>SSSTTLHNAMQYTAFDVLSSILNLMKADPLYDLLQLNQAYSSQDQEYEKNEFYGDSYLEERASSLVLKFLRKYEQIPFEMYSGLRIHTVKNQTLGEIFDLLHLGDTKTFEKKKKGDLVESLIGGCVLLSQRENATLFLLFAHALIDYIFYHSSYIY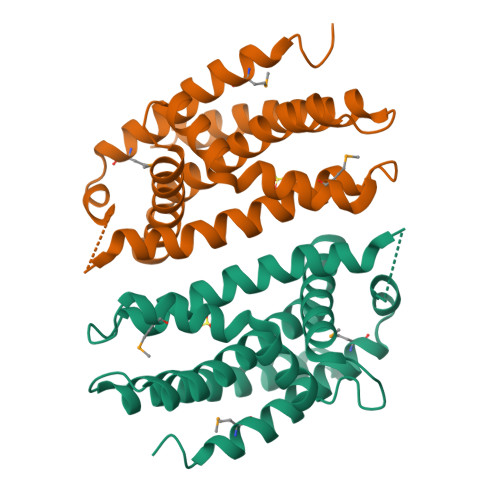FNANPPKLVKEEIITDIQNWFKDKLFYYRSSLEKYQT[2x]>MENKVVEEKQVDKIPLMSPCKMGKFELCHRVVLAPLTRQRSYGYIPQPHAILHYSQRSTNGGLLIGEATVISETGIGYKDVPGIWTKEQVEAWKPIVDAVHAKGGIFFCQIWHVGRVSNKDFQPNGEDPISCTDRGLTPQIMSNGIDIAHFTRPRRLTTDEIPQIVNEFRVAARNAIEAGFDGVEIHGAHGYLIDQFMKDQVNDRSDKYGGSLENRCRFALEIVEAVANEIGSDRVGIRISPFAHYNEAGDTNPTALGLYMVESLNKYDLAYCHVVEPRMKTAWEKIECTESLVPMRKAYKGTFIVAGGYDREDGNRALIEDRADLVAYGRLFISNPDLPKRFELN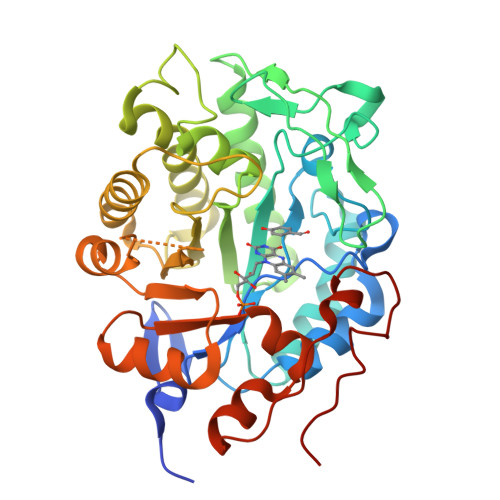APLNKYNRDTFYTSDPIVGYTDYPFLETMT[2x]>CTDAALAALEYHKSNA[18x];>CVSMIGGSR[18x];>RVSIGGTVYTAKKYDD[18x];>[18x]PFGAD;>[18x]MMAEHDQNNDEYKFAELDSYDMDQAGESDLDSEASYQSGKEGLTKKKDIKRNALIAIGAVVFIMVMYKIIGWMFFSDKSSQVTSKPAIPPVTQVATPQPVQTIPTTTPIQQVQPTTIIEDDPDLKKKVSAIEMTQQSLRSEVNALSEQINAVNNNIKNLNAQIVNLNQIIGNMSNQIARQSEVINVLMARTTPKKVVKVSRPIVQARIIYYIQAVIPGRAWLIGSNGSTLTVREGSKIPGYGMVKLIDSLQGRILTSSGQVIKFSQEDS;>MMKKYDQLCKYCLVIGLTFSMSCSIYAADQSDDAQQALQQLRMLQQKLSQNPSPDAQSGAGDGGDNAASDSTQQPNQSGQANAPAANQTATAGGDGQIISQDDAEVIDKKAFKDMTRNLYPLNPEQVVKLKQIYETSEYAKAATPGTPPKPTATSQFVNLSPGSTPPVIRLSQGFVSSLVFLDSTGAPWPIAAYDLGDPSSFNIQWDKTSNTLMIQATKLYNYGNLAVRLRGLNTPVMLTLIPGQKAVDYRVDLRVQGYGPNAKSMPTEEGIPPSANDLLLHVLEGVPPPGSRRLVVSGGDARAWLSNEKMYVRTNLTILSPGWLASMTSADGTHAYEMQKSPVLLVSWHGKVMQLKVEGL[18x];>[23x]MASKKENLKSLFSNTRTRVIIIFTAALLIIAVVIGFFKIRGATTGSIAAAEVSTVPGGIQSIPGVLDPTAQYAKLQEEQNITQAQVAEKTGGSAIPTIIRTQALGEGVGVIGSQSGVGFAALAQEELGGPQRSLWIQELQDGSCSKSVITKVVNQGAQLTDLKAACSCVQLKDSGYGLQELEQVCECKELKSAGYNARQLKEAGYSAGRLRNCGFDACELRNAGFTAQEMKDGGFSDGELKGAGFSDAEIAKASGLPDGITADDVRKAGCGAAALAKLRQAGVSASAIRKISGCTAEQLKAAGYTAKELKDAGFSAADLRRAGFSAAELKDAGFTARDLLNAGFTPADLAKAGFSDAQIKAAQAELPPGITPQDVKNAGCDVEALKKEREAGVSAALIRQYAGCSAQALKAAGFTDADLANAGFTPAQISAATPLSDAEIKAAGCDPDKLKKLFSAGVSAKRIKELNGCSAEALKAAGYDAQSLLAAGFTPQELLAAGFTPKQLEDAGLNPVSIIADGRVADCSVESLKKARAAGVSALTIKQTLGCSAAALKAAGYTAKELKDAGFTAAELKAAGFSAKELKDAGFTAKELRDAGFSAQELKDVGFSAKDLKDAGFSAAELKAAGFTAAQLKAAGFSAKDLKDAGFSAAELKAAGFSAKELKDAGFSASDLKNAGFSAKELKDAGFSASDLKSAGFSASELKNAGYSADELKKAGYTSAELRNAGFSPQESAVAGLQGPDLQQLDSSITGIPSIPGATPRPTTSDAASSAEQLQAILQKQNEQLAEQKYQQEIQQRTSDMLTAATQLVQDWKQVETQVYTEGTEETKTSGGESAVPGTGTGTGSNNQPVDQGAVSAQNQAIIKTGDIMFAVLDTSVNSDEPGPILATIVTGKLKGSKLIGSFNLPSNADKMVITFNTMSIPGAEKTISISAYAIDPNTARTALASRTNHHYLMRYGSLFASSFLQGFGNAFQSANTTITIGGTGGGNNITVANGVGRSTLENAVIGLATVGKAWSQQAQQLFNTPTTVEVYSGTGLGILFTQDVTTI;>MKVLPKLALANLVCFTTLSVFAQPADPSGQQTSTNTSNLVTYLTNLGKYLGYDITQSSKAPNPPYSQLFNSNVVQLVQNYAYNTFLGAIPVDAMSQSLMNFVTDKVQGNSLINNLANTTFKYQNFSAPSSGADGKITANGLIDQSTASAQTPTTPGIFSAPQITTSGTYLNDPVSQAVFNILGTPDYSFCMDNEQKNWLPNCNLMYQNLVMQNVIGTLPPAQTSGSTPAFYSYKYNQPLISQLNSNSLIAPLLMDTSASQSGQDSGLTAKSQAQQALNFIRYASAQVTPPSLPKLSAYSELWNQATAKPNSAGYNEVQQKQAAATLSSYFNNLRVYAAQTSVGVSNLYYILSKRLPQNMSADQSNANITSQALNEFNMATRRLFDPTASNTPGQPNQQWIKQINDASPATVQKEIAILLAEINYQMYLDRQIQERILLTNSIMLLQNLKAAQPTADFSSQGSPSEQ[5x];>MNKLAITVLLCFFPALALAENGALSFAPPASDLSVVFLGNLFGVVDGVLHGTGSQIMGNMFGVFNSAVLALGGIIIMYTLMVSTMNTAHEGQMLGQKWSSIWIPLRSTFGLALLIPKASGYCMMQVFFMWVIVQGVGAADKIWEAALSYLNRGGVIIQAQADPTKSLQAAGSSSSGVAKGALTILGGQICMLGLQKQLQAQRDLYLSQSKSPPCGGNPTPEMNTFCRTAIPDFISTVNFVKKQNDDTPKDLTANQPA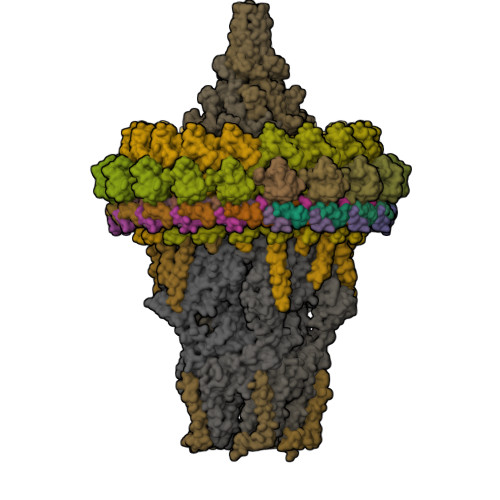SFELDMPNFDKSSPFYFLNGICGTVKWNNISALNSTNQSDNKGLVTVGGAGSNSSMGANSLNITSSQLQTARLSRAIAIQQMYVTLSTVAQVMVNNDPAFSTTTSTGNSKNDFSAIAKQQFGVPYKSSGEVCTEYQQVCQTWGSVPSSTGSTTGVLFNGTEFLGAINDYNGIMMPTLNLIRQATSKEFDKKSRDFIAEANAKGWIMAGSYFFDLVKLNGSATEFADQFDTGTGLDKSSFDPTQLTKPFGKTCQDPYSLLCTWFQNKSDKLIQIQSLIDGVPALGQDGVKQPDLSDNPQRQSVSGPLSSTVYGFVNNSMMVQLPGQPGIKPLTFANLINFKVDTSLYYMKHQDFDCGRVKILFFSFCLGRMMGDLFYNYVFRYVYNFFLAIFGEMINSIVMAFLMIPLQGMKDIFIVGVQTLTQPGINPIVALANMGTMYINFSGTLWLTLLNMAVVSSLIPLFGIFIFALIMMAMPLLMAWIGTMVSIGFVTAYYIPVLPYMIFTFGSFAWLIAVIEAMVAAPIVALGVTHPEGNEAFGKGEFAIMILVNVFLRPSLMIIGYIAAIALSYVGVWILNAGFDHAISYIQSDQGIETWEKGTSSNDAKRFFQSAGNWTGAKMDTSQWDNFKDKLTGDYQSTALEGGYTGWAGVYAFFFSILIYTSMYLIIVQKAFTLIAHLPDKVLRWIGGSPESFGQETMQWGEEAKGRVEKAGEATYGAEKAIGDKLGAKGQEMLGKLGPQAKKISENAGDVSGKGKNSGGSQTGPSSKPDTGQQLGGSDSGTPTSTPPPE[5x]> MNSLSEANTKFMFDLFQQFRKSKENNIFYSPISITSALGMVLLGAKDNTAQQIKKVLHFDQVTENTTGKAATYHVDRSGNVHHQFQKLLTEFNKSTDAYELKIANKLFGEKTYLFLQEYLDAIKKFYQTSVESVDFANAPEESRKKINSWVESQTNEKIKNLIPEGNIGSNTTLVLVNAIYFK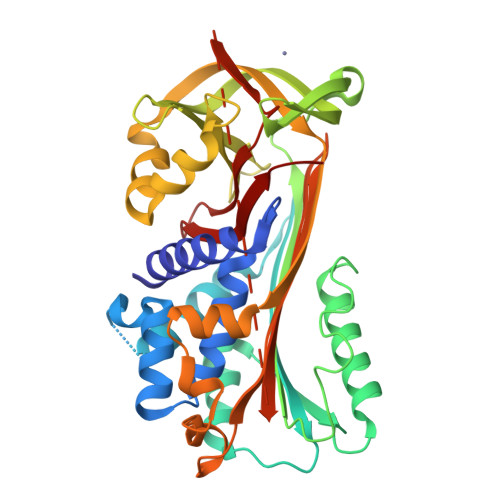GQWEKKFNKEDTKEEKFWPNKNTYKSIQMMRQYTSFHFASLEDVQAKVLEIPYKGKDLSMIVLLPNEIDGLQKLEEKLTAEKLMEWTSLQNMRETRVDLHLPRFKVEESYDLKDTLRTMGMVDIFNGDADLSGMTGSRGLVLSGVLHKAFVEVTEEGAEAAAATAVVGFGSSPTSTNEEFHCNHPFLFFIRQNKTNSILFYGRFSSP>[2x]GPGSMSEEAFIYEAIRTPRGKQKNGSLTEVKPLNLVVGLVDELRRRYPDLDETLISDMILGVVSPVGDQGGDIARTAVLAAGLPETTGGVQLNRFCASGLEAVNTAAQK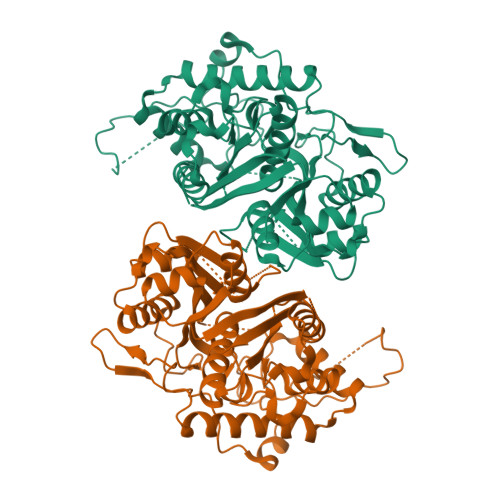VRSGWDDLVLAGGVESMSRVPMGSDGGAWATDPETNYRIGFVPQGIGADLIATLEGFSREDVDAYALRSQQKAAAAWSGGYFAKSVVPVRDQNGLVILDHDEHMRPDTTMEGLAKLKTAFDGVGEMGGFDDVALQKYHWVEKINHVHTGGNSSGIVDGAALVLVGSEKAGKSQGLTPRARIVATATSGSDPVIMLTGPTPATRKVLDRAGLTIDDIDLFELNEAFASVVLKFQKDLNIPDEKLNVNGGAIAMGHPLGATGAMITGTMVDELERRNARRALITLCIGGGMGVATIIERV>[2x]MSLDRQLWRQFPQVEPQLTALQDYLLRTVQLDNQPIHHKILALLKSGGKLLRPGYFYLFSTFGNAATPAQLQAGAAAIEILHVGTLIHDDVIDDSPTRRGVRTIQMTYGQRNAIYAGDFMFTVYFDQVLKSTTDRSLIQNHIDAMHRILQGELHQMDLNYREDITLDAYLNEIAGKTAELFALSCYQGAQLAGAPQSVIDRTRDIGIAIGCAYQMLDDILDYAGDPKRTQKPVLEDLRSGVYSLPLLLS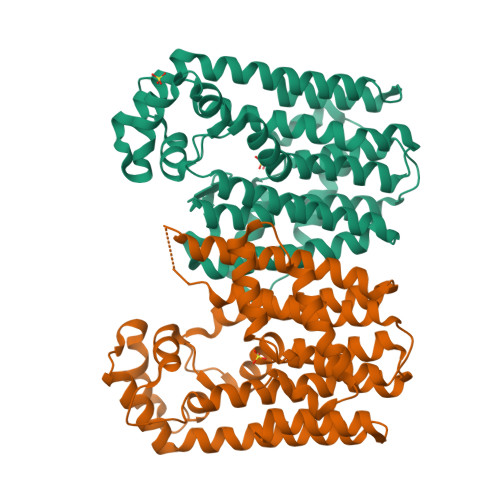LSHAPRDFHKLLKKKQAMTLEDIKHVQALVAQYDGVGAAKQLAQDYTDRALTLIQQLPVGSAQQSLEQLTRLLLRRDHEGHHHHHH>[4x]GAPPAPALRIDYPKALQILTEGGTHMVCTGRTHTDRLCRFKWLCYSSEAEEFIFFHGNASVMLPSLGSRRFQPALLDLSTVEDHNTQYFNFVELPAAALRFMPKPVFVPDVALIANRFNPDNLMHVFHDDLLPLFYTLRQFPGLAREARLFFMEGWGEGAHFDLYKLLSPKQPLLRAQLKALGRLLCFSHAFVGLSKVTTWYQYGFVQPQGPKANILVSGNEIRQFAHFLMEKLNVSQAGGPLGEEYILVFSRTQNRLILNEAELLLALAQEFQMKT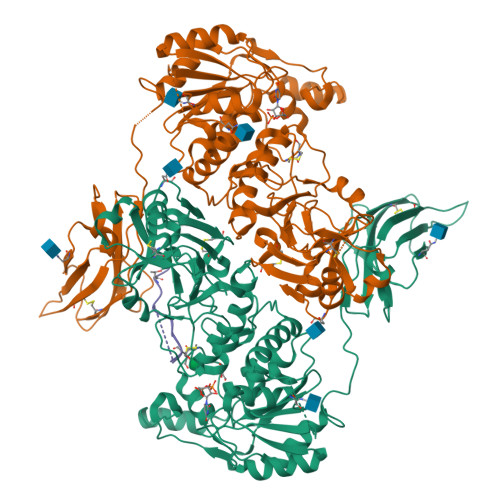VTVSLEDHAFADVVRLVSNASMLVSMHGAQLVTALFLPRGAAVVELFPYAVNPDHYTPYKTLATLPGMDLQYIAWQNTMPENTVTHPERPWDQGGIAHLDRAEQARILQSREVPRHLCCRNPEWLFRIYQDTKVDIPSLIQTIRRVVKGHPGPRKQKWTVSLYPGKVREARCQASVQGASEARLSVSWQIPWNLKYLKVREVKYEVWLQEQGENTYVPYMLALQNHTFTENIKPFTTYLVWIRCIFNKTLLGPFADVLVCST;>XTIRTRGAIIQTPTLGPIQPTRX[2x]> MINRSTAFISKNLRQANLTQSSLAMKTQYNQMGFSSDNPYNKRWEYKWKHSYYTYPRDYEHTEVRKPQDSKDVPPIYFAYYKDFVDRWLPGMNMWWQRRHRIFDKFNVYFLPGMSLFFYQFADLALGFKIMAAFPLFLAYTRIRDKTLDPDFKETYLRDMIYQNPEITKYFNEETIHVLDYEFEYLPGYLCPEKFPEYQNKTWQFFNTDTAQAEGFFKFGDVESGATMTLKFKTMPIPGKFRYQVGEPFYFYDLRAEIKCDGV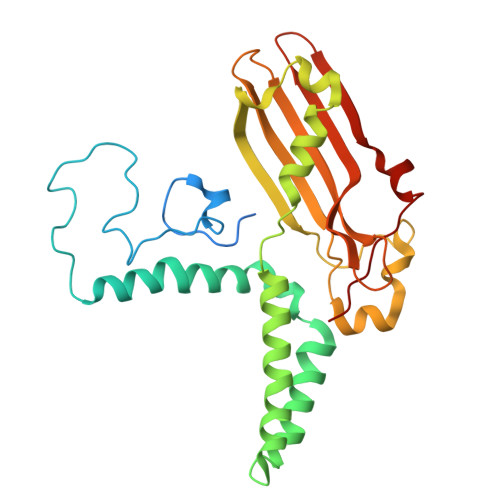YKEVVLVDEKESLKKIRPFLFLI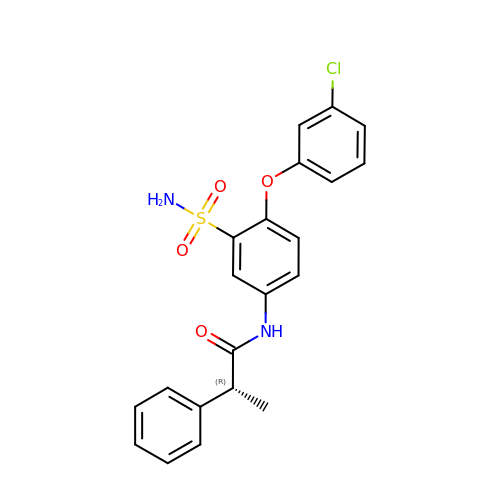(2~{R})-~{N}-[4-(3-chloranylphenoxy)-3-sulfamoyl-phenyl]-2-phenyl-propanamide | C21 H19 Cl N2 O4 S | QEACKKQHBTVOBS-CQSZACIVSA-N ethyl 3,5-dimethyl-4-{[4-(trifluoromethyl)phenyl]methyl}-1H-pyrrole-2-carboxylate 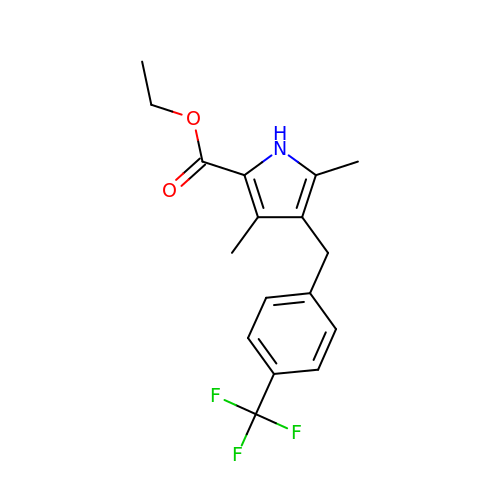| C17 H18 F3 N O2 | PWRCYLHLZGCFQH-UHFFFAOYSA-N>[3x]GHMNKSEISQVFEIALKRN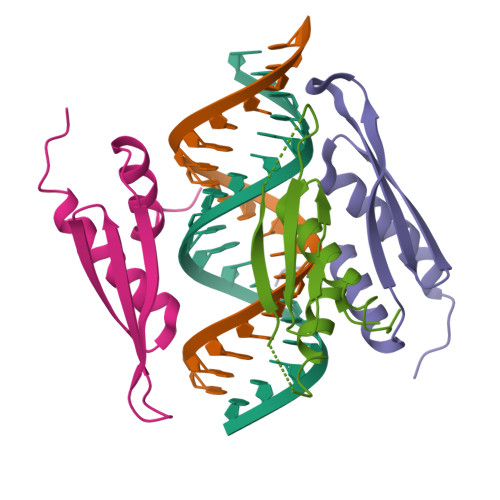LPVNFEVARESGPPHMKNFVTKVSVGEFVGEGEGKSKKISKKNAAIAVLEELKKLPPLPAVERVKPRIKKKTKPIVKPQTSPEYGQGINPISRLAQIQQAKKEKEPEYTLLTERGLPRRREFVMQVKVGNHTAEGTGTNKKVAKRNAAENMLEILGFKVPQRQ>MAAAVVLAAGLRAARRAVAATGVRGGQVRGAAGVTDGNEVAKAQQATPGGAAPTIFSRILDKSLPADILYEDQQCLVFRDVAPQAPVHFLVIPKKPIPRISQAEEEDQQLLGHLLLVAKQ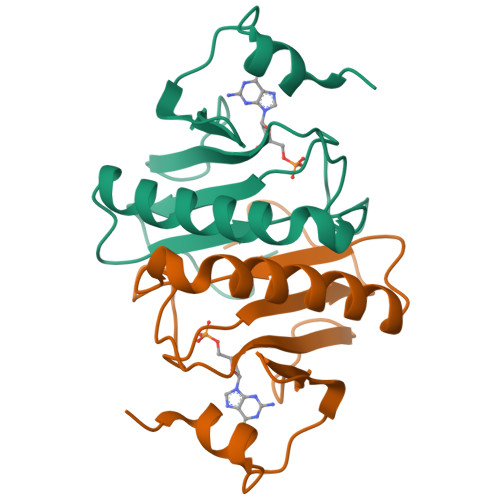TAKAEGLGDGYRLVINDGKLGAQSVYHLHIHVLGGRQLQWPPG[2x]2-[3,6-bis(dimethylamino)xanthen-9-yl]-5-methanoyl-benzoate | 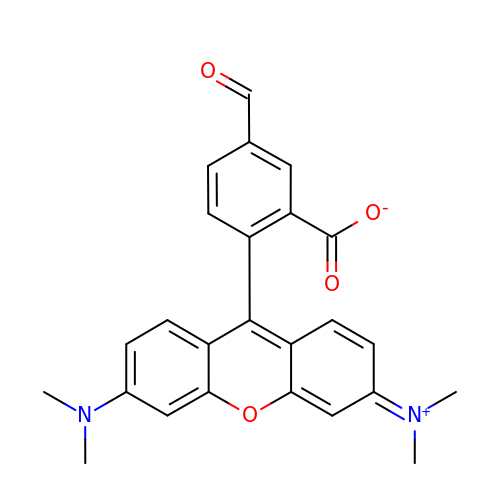C25 H22 N2 O4 | ZFGLYCCNMJCDCP-UHFFFAOYSA-N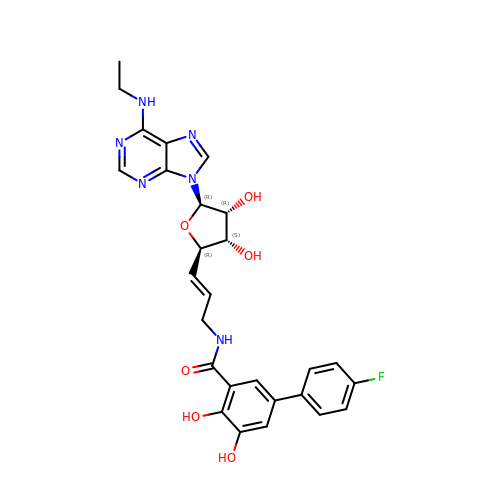N-[(E)-3-[(2R,3S,4R,5R)-5-(6-ethylaminopurin-9-yl)-3,4-dihydroxy-oxolan-2-yl]prop-2-enyl]-5-(4-fluorophenyl)-2,3-dihydroxy-benzamide | C27 H27 F N6 O6 | NOCNCHHJBSJZFZ-CJLJSIFTSA-N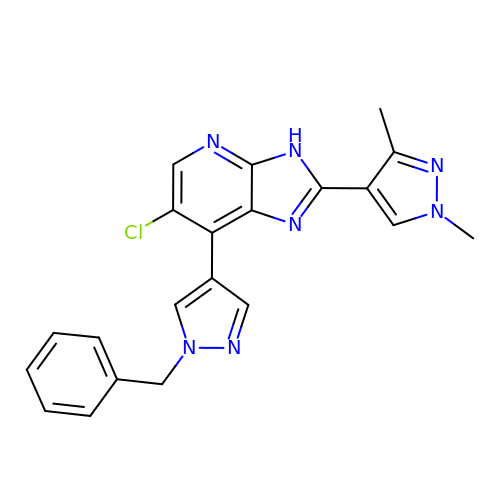7-(1-benzyl-1H-pyrazol-4-yl)-6-chloro-2-(1,3-dimethyl-1H-pyrazol-4-yl)-3H-imidazo[4,5-b]pyridine | C21 H18 Cl N7 | IDYBEIZHMAGVLB-UHFFFAOYSA-N(2S,3R,5S)-5-(6-amino-9H-purin-9-yl)-tetrahydro-2-(hydroxymethyl)furan-3-ol | C10 H13 N5 O3 | 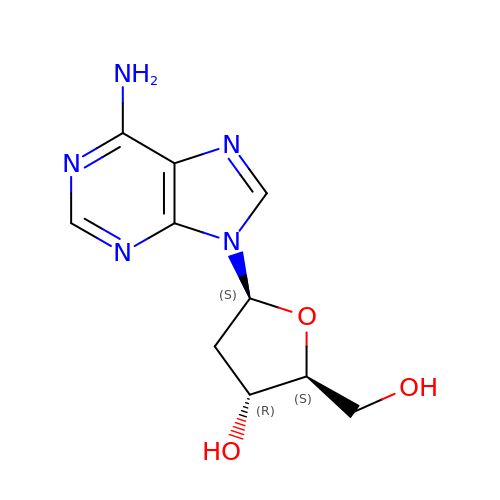OLXZPDWKRNYJJZ-VQVTYTSYSA-N> MVARVQTAEEIRDEGNAAVKDQDYIKADELYTEALQLTTDEDKALRPVLYRNRAMARLKRDDFEGAQSDCTKALEFDGADVKALFRRSLAREQLGNVGPAFQDAKEALRLSPNDKGIVEVLQRLVKANNDKIKQTTSLANKVTDMEKLAFRGEAKDTEQKMTALNNLLVLCRESESGATGVWNQGALVPFVLNLINDASENEEVTVTAIRILDETIKNSVRCMKFLAMHDPDGPKSVRFVCRLMCKKSTKDFVDATGILVQRVFNAMAKMDRQKEMKPDPEVAEANKIWIIRVLLELQEMLQDPKVGAVQRETCIDLFLKNLMHMDGGIPRGWSWKFVEERGLLALLDVASQIPELCEYPVSAETRQHVAICLQRLEEDMVFDTKRTIFKEKVDMFFNALISRCTNDDEGHKYRIKLSCFLITMLQGPVDIGINLITNDQLTPIMLEMAASQDHLMQGIAAELIVATVSKHERAINMLKVGIPVLRALYDSEDPTVKVRALVGLCKIGAAGGDDISKATMKEEAVISLAKTCKKFLLETEKYSVDIRRYACEGLSYLSLDADVKEWIVDDSLLLKALVLLAKKAGALCVYTLATIYANLSNAFEKPKVDEEMVKLAQFAKHHVPETHPKDTEEYVEKRVRALVEEGAVPACVAVSKTESKNALELIARSLLAFAEYEDLRGRIIAEGGTVLCLRLTKEASGEGKIKAGHAIAKLGAKADPMISFPGQRAYEVVKPLCDLLHPDVEGKANYDSLLTLTNLASVSDSIRGRILKEKAIPKIEEFWFMTDHEHLRAAAAELLLNLLFFEKFYEETVAPGTDRLKFWVLYSAEVEEERLSRASAAGFAILTEDENACARIMDEIKSWPEVFKDIAMHEDAETQRRGLMGIANIMHSSNKLCSEIVSSEVFRVLVAVTKLGTINQERAG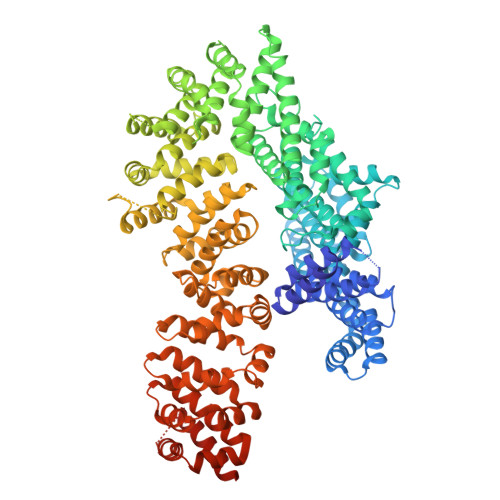STEQAKRGLEAAEKFGLIKATDREIYERENQMSTIQE> XEHF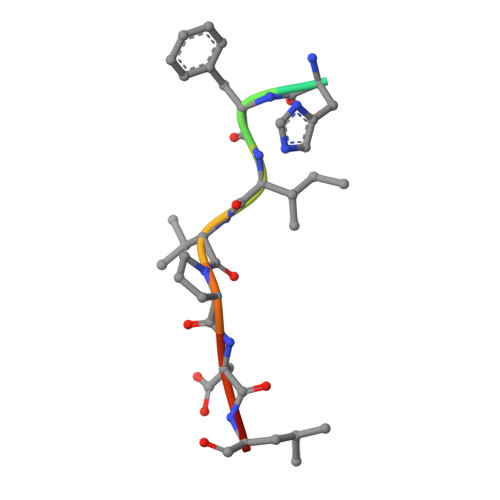IVPDLY> MNLPTAQEVQGLMARFIELVDVGDI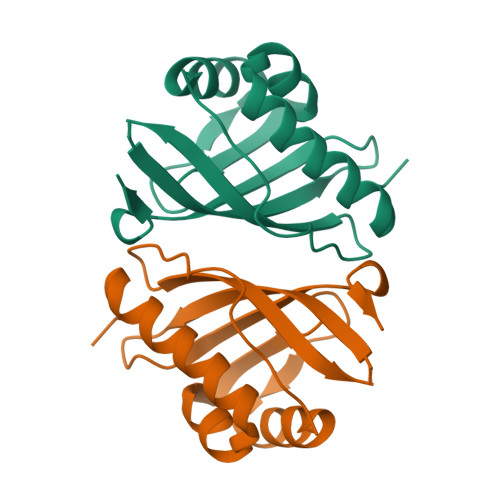EAIVQMYADDATVEDPFGQPPIHGREQIAAFYRQGLGGGKVRACLTGPVRASHNGCGAMPFRVEMVWNGQPCALDVILVMRFDEHGRIQTMQAYWSEVNLSVREPQ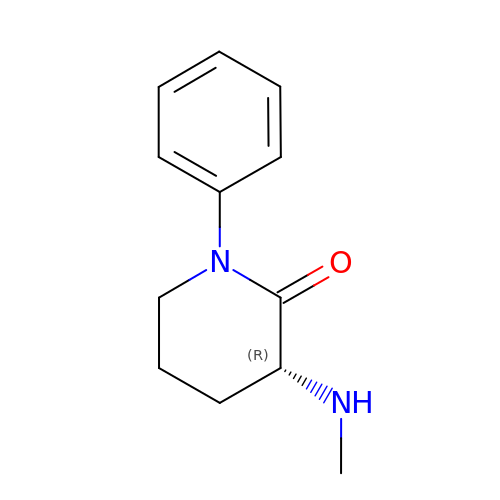(3R)-3-(methylamino)-1-phenylpiperidin-2-one | C12 H16 N2 O | PVGKKAFLCYRCCI-LLVKDONJSA-N>ADKELKFLVVDDQSTMRRIVRNLLKELGFNNVEEAEDGVDALNKLQAGGYGFVISDWKMPNMD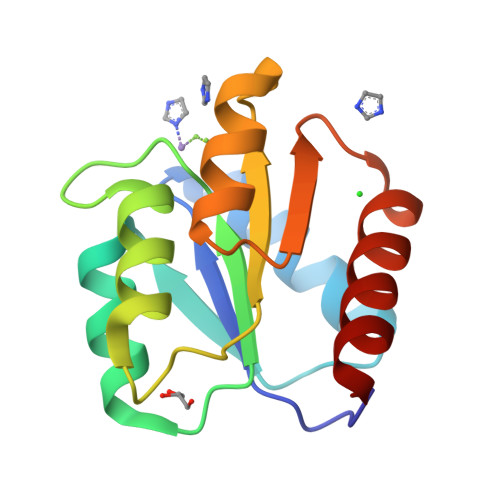GLELLKTIRADGAMSALPVLMVTAYAKKENIIAAAQAGASGYVVKPFTAATLEEKLNKIFEKLGM[2x]>MSLTSSAELAEVDTLARSLLLYRSRLAEYAHANPGFSGSPADSALGLPAWFRKPVRLQGYIAAGTSYAFIASPPAGLAAAVDT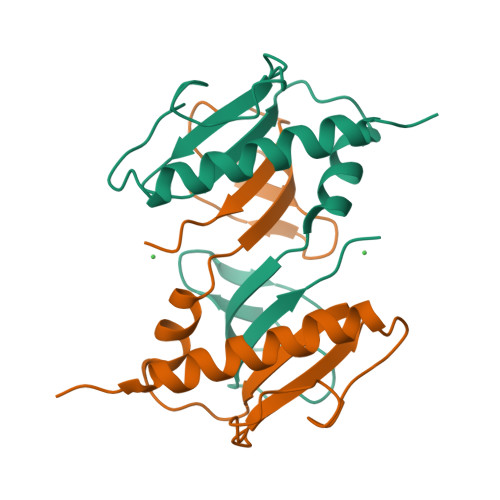GTESDLVGVRRNGQLVTRRLGATAIALPAPIPEGAVVAVKEGHHHHHH[2x]>[4x]MDPEFTNLIHFQSTEGKIWLGEQRMLLLQVSAMASFRREMVNTLGIERAKGFFLRQGYQSGLKDAELARKLRPNASEYDMFLAGPQLHSLKGLVKVRPTEVDIDKESGRFYAEMEWIDSFEVEISQTDLGQMQDPVCWTLLGYACAYSSAFMGREIIFKEVSCRGCGGDKCRVIGKPAEEWDDVASFKQYFKNDPIIEELYELQSQLVSLRTNLDKQEGQYYGIGQTPAYQTVRNMMDKAAQGKVSVLLLGETGVGKEVIARSVHLRSKRAAEPFVAVNCAAIPPDLIESELFGVEKGAFTGATQSRMGRFERADKGTIFLDEVIELSPRAQASLLRVLQEGELERVGDNRTRKIDVRVIAATHEDLAEAVKAGRFRADLYYRLNVFPVAIPALRERREDIPLLVEHFLQRFHQEYGKRTLGLSDKALEACLHYSWPGNIRELENVIERGIILTDPNESISVQALFPRA

The bacterial enhancer binding (bEBP) subgroup of AAA+ proteins couple ATPase hydrolysis to initiation of transcription by σ54-RNA polymerase (σ54-RNAP). DmpR (di-methyl phenol regulator) from Pseudomonas putida KCTC 1452 (also known as CapR) is a single-component bEBP that serves as a sensor of phenolic compounds. As is typical of bEBPs, DmpR consists of three domains: (1) a sensory domain consisting of a vinyl-4-reductase (V4R) scaffold that functions in binding of an aromatic effector molecule, (2) a conserved central AAA+ ATPase domain bearing the bEBP-specific GAFTGA motif that is involved in coupling ATP hydrolysis to the restructuring of σ54-RNAP, and (3) a DNA binding domain that interacts with the palindromic upstream activating sites (UASs) situated ~100–200 bp upstream from the σ54 promoter. DmpR share high sequence homology with other aromatic-responsive bEBPs, such as XylR, TouR, PoxR and MopR, and this subgroup are known to transition from inactive dimers to active oligomers upon the binding of an aromatic effector compound as a prerequisite for their capacity to direct σ54-dependent transcription.

Based on a solubility profile analysis and preliminary tests, we designed a truncated DmpR derivative (aa 18–481) that is soluble and produced at sufficient levels in E. coli. This truncated protein, DmpRΔD, has an N-terminal 6 × His tag that replaces the first 15 residues, lacks the DNA binding domain, and carries serine substitutions of two cysteine residues (C119S/C137S) that were anticipated to be located at the protein surface. The determined crystal structure of DmpRΔD shows a phenol molecule bound to the sensory domain of each protomer. The DmpRΔD-phenol complex is a dimer-of-dimers with overall dimensions of 150 × 75 × 70 Å. The two protomers (P1 and P2) form an elongated intertwined P1/P2 dimer through extensive interactions between the related sensory domains and parallel coiled-coil B-linkers in a head-to-head orientation with a buried surface area of 2895 Å2. The two dimers—P1/P2 and P3/P4—form the tetramer, which has an antiparallel head-to-tail assembly that places the four ATPase domains at the central core of the complex. The P1/P2 sensory domain dimer packs against the ATPase domains in the P3/P4 dimer in such a way that the Val53 and Ile58 residues in the P1 sensory domain interact with Phe312 in the GAFTGA motif (aa 310–315) in the P3 ATPase domain. The phenol is located in an enclosed cavity (24–36 Å3 in volume) formed by an antiparallel hairpin motif. A strictly conserved Trp128 residue is located between the phenol-binding site and the zinc-binding site, while the zinc is coordinated by residues Cys151, Glu172, Cys177 and Cys185. Interestingly, the electron density of the phenol group is strong in the P1 protomer, whereas it is weak in the P2 protomer.> GPGSMEALVRALEEADHAVATVVQSRILEFFMAAGRETPAGVRGLWARALRLACRAYVETGTCEAAVLAENLAGLALWRLRHDWDEGTAPLLELLGVVNGDDTTAALTEAGLRTSAEFGPDAMFRLVSEWCAAFDEALAGARSADDVLAAPRVVPPEQTARALVQPRFATLYDMDFVQDGLRYVAQHTNWALPLALAVRQMQNEGLKPLTRALFALTIADEFFHDRQNPTLREQFAEAARAVDEAALVPVGEVNATPRTAVEVRVSAALAHGDAYVRELRPGTVARRLRTDQGVLALLDPGAQAVHVAAAADLDHTQVDATGVWEAVAASASPLQVVEALVTAGFTRRHCDLLERAVLDRAPRLTAAQAAVGCTAVVGGVVHRLLDDYGPGLDYVRAYTDVADTLEPLYGDVTAALGLPEKGVEAVVRACMAPRPPTEHVGAARAALLREVAAAERRAGLAHSAAREALNTWLAFRAQSRWGLRADGAGETPMEAPTSAA

Although the majority of the tegument disassociates from the capsid at this stage, three tegument proteins remain capsid bound: pUL36, pUL37, and pUS3. Like pUL36, pUL37 promotes translocation of incoming capsids to the nucleus. We recently determined the crystal structure of the N-terminal half of pUL37 and identified three evolutionarily conserved surface-exposed regions: R1, R2 and R3. Our results indicate that the conserved R2 region in the pUL37 inner tegument protein rectifies this motion to produce sustained retrograde bias.

We previously mutated three evolutionary conserved surface regions of the pUL37 tegument protein (R1, R2, R3) in PRV. Each mutated region consisted of five alanine substitutions. Although plaques produced by the R2 mutant were smaller than wild type, all three mutants propagated to wild-type titers. Remarkably, the R2 mutant was avirulent despite propagating to wild-type titers in culture. To determine if the stark R2 mutant phenotype resulted from misfolding of the mutant pUL37 protein, the crystal structure of the pUL37 N-terminus was solved and overlaid with the previous WT structure. The five point mutations did not affect the overall fold of the N-terminal half of pUL37 as judged by the alignment of the wild-type and R2 mutant crystal structures (rmsd = 0.55 Å). These findings demonstrated that introduction of the mutations did not contort the pUL37 backbone, and encouraged us to further examine the R2 mutant in cell culture infection models to identify the specific source of its avirulence. Whereas wild-type HSV-1 and PRV capsids preferentially moved in the retrograde direction in axons (towards the neural soma), capsids of the R2 mutants moved in an aberrant bidirectional manner best described as “ping-ponging”. Firstly, the PRV R2 mutant failed to spread to the TG following inoculation into the anterior chamber of the eye, which was consistent with the HSV-1 R2 mutant defect in vivo, and pinpointed R2 as a conserved effector of alpha-herpesvirus neuroinvasion. Taken together, the in vivo studies recapitulated the results obtained with primary cultured sensory neurons: R2 is required for retrograde axonal transport but is dispensable for anterograde axonal transport.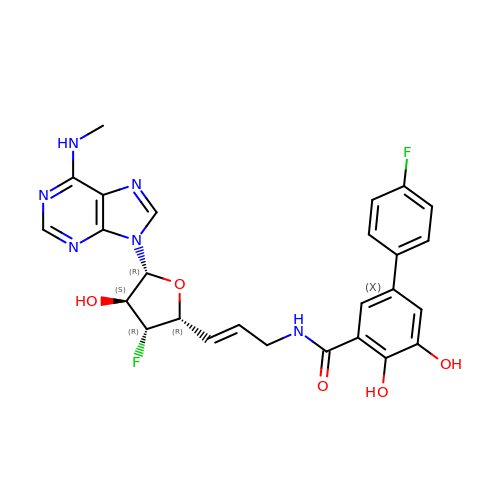N-[(E)-3-[(2R,3R,4S,5R)-3-fluoro-4-hydroxy-5-[6-(methylamino)purin-9-yl]oxolan-2-yl]prop-2-enyl]-5-(4-fluorophenyl)-2,3-dihydroxy-benzamide | C26 H24 F2 N6 O5 | ZHVVVGDBOITDFN-UJYAWEMASA-N Rather, it exists as a stable heterotrimer in which the apo-enzyme PolB1 associates with two subunits that we term PolB1-binding protein (PBP) 1 and PBP2. The PBP1 and PBP2 proteins are conserved in the Sulfolobales and other members of the crenarchaeal phylum and so, since the majority of our studies of the replisome have been performed with proteins from Sso, we chose to study the Sso orthologues, the products of the SSO0150 (PBP1) and SSO6202 (PBP2) open reading frames. In conclusion, over 30 years after its first characterization, we reveal that Sulfolobus PolB1 is not a single-subunit enzyme as was previously believed, but rather is a heterotrimeric holoenzyme. We speculate that PBP2 may facilitate polymerase activity via its interactions with the knuckle on the thumb domain of PolB1, conceivably influencing the position of the tip of the thumb domain and modulating the interaction of this domain of PolB1 with the primer–template junction.

PBP2 was crystallized and the structure determined by multiple wavelength anomalous dispersion (MAD) phasing technique. We note, however, that we cannot detect any direct interactions between PBP2 and either single- or double-stranded DNA.

> MSVNQKEIEIAIEYFKNYISVGEIVATMDLKARGISNPQAVISKLIEMGIIEKGEGCYNLVRKSTDKKLEHHHHHH>[2x]MKNMPENHNPQANAWTAEFPPEMSYVVFAQIGIQSKSLDHAAEHLGMMKKSFDLRTGPKHVDRALHQGADGYQDSIFLAYWDEPATFKSWVADPEVQKWWSGK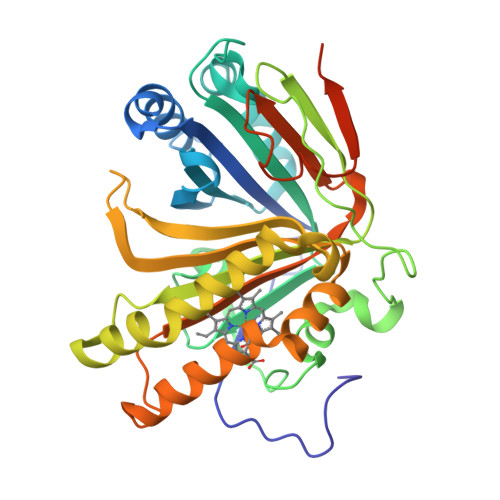KIDENSPIGYWSEVTTIPIDHFETLHSGENYDNGVSHFVPIKHTEVHEYWGAMRDRMPVSASSDLESPLGLQLPEPIVRESFGKRLKVTAPDNICLIRTAQNWSKCGSGERETYIGLVEPTLIKANTFLRENASETGCISSKLVYEQTHDGEIVDKSCVIGYYLSMGHLERWTHDHPTHKAIYGTFYEMLKRHDFKTELALWHEVSVLQSKDIELIYVNCHPSTGFLPFFEVTEIQEPLLKSPSVRIQKLAAALEHHHHHH>[2x]EHAERLPYDASKWEFPRDRLKLGKPLGRGAFGQVIEADAFGIDKTATCRTVAVKMLKEGATHSEHRALMSELKILIHIGHHLNVVNLLGACTKPGGPLMVIVEFCKFGNLSTYLRSKRNEFVPYKVAPEDLYKDFLTLEHLICYSFQVAKGMEFLASRKCIHRDLAARNILLSEKNVVKICDFGLARDIYKDPDYVRKGDARLPLKWMAPETIFDRVYTIQSDVWSFGVLLWEIFSLGASPYP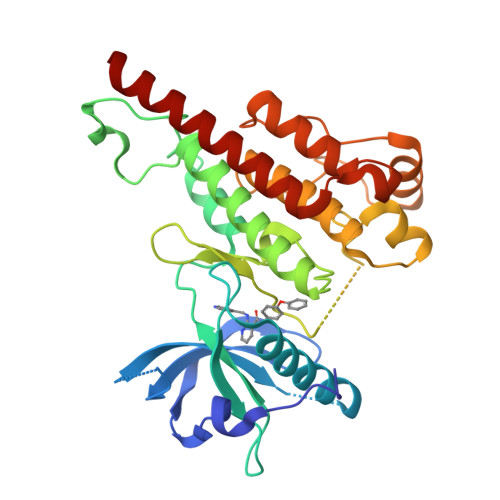GVKIDEEFCRRLKEGTRMRAPDYTTPEMYQTMLDCWHGEPSQRPTFSELVEHLGNLLQANAQQDRHHHHHH3-[2-bromanyl-4-(trifluoromethyl)phenoxy]-N-methyl-3-phenyl-propan-1-amine | C17 H17 Br F3 N O | 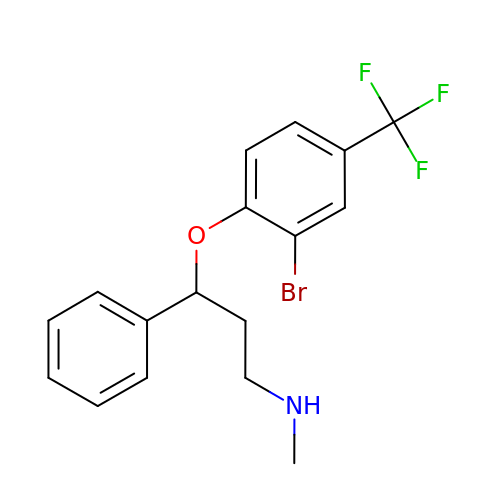KZCOQBCCEHGWOG-UHFFFAOYSA-N> HHHHHHEQKLISEEDLEGIKYRRNELFLDVLESVNLLMSPQGQVLSAHVSGRVVMKSYLSGMPECKFGMNDKIVIEKQGKGTADETSKSGKQSIAIDDCTFHQCVRLSKFDSERSISFIPPDGEFELMRYRTTKDIILPFRVIPLVREVGRTKLEVKVVIKSNFKPSLLAQKIEVRIPTPLNTSGVQVICMKGKAKYKASENAIVWKIKRM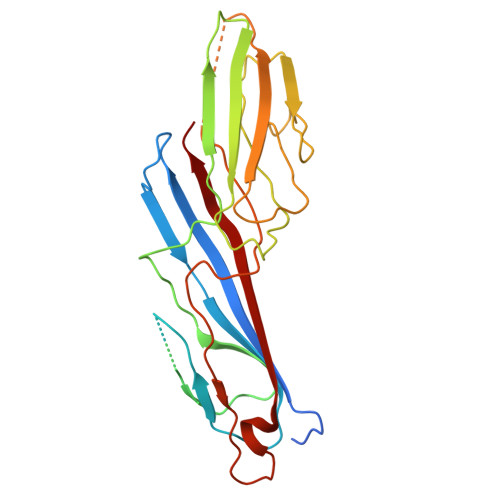AGMKESQISAEIELLPTNDKKKWARPPISMNFEVPFAPSGLKVRYLKVFEPKLNYSDHDVIKWVRYIGRSGIYETRC[(1~{S},2~{R})-1-[1-(1,3-benzodioxol-5-ylmethyl)-1,2,3,4-tetrazol-5-yl]-3-(4-~{tert}-butylphenyl)-2-methyl-propyl]diazane | 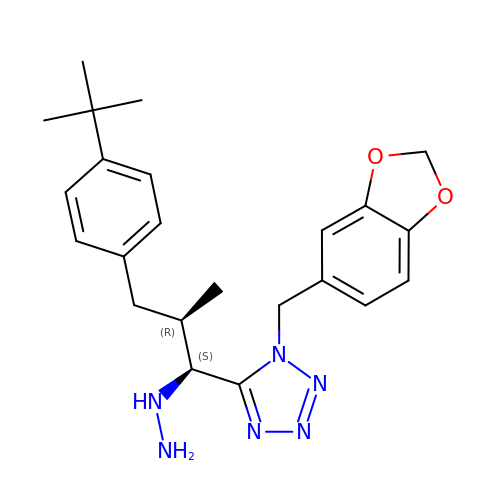C23 H30 N6 O2 | BBOIZOIQFPNBML-VFNWGFHPSA-N> NECLGTIGPVTPLDASDFALDIRMPGVTPKESDTYFCMSMRLPVDEEAFVIDFKPRASMDTVHHMLLFGCNMPSSTGSYWFCDEGTCTDKANILYAWARNAPPTRLPKGVGFRVGGETGSKYFVLQVHYGDISAFRDNHKDCSGVSVHLTRVPQPLI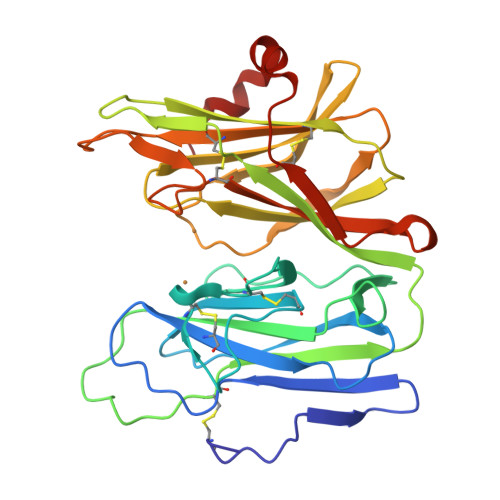AGMYLMMSVDTVIPPGEKVVNADISCQYKMYPMHVFAYRVHTHHLGKVVSGYRVRNGQWTLIGRQNPQLPQAFYPVEHPVDVTFGDILAARCVFTGEGRTEATHIGGTSSDEMCNLYIMYYMEAKYALSFMTCTKNVAPDMFRTIPAEANIPIP>[6x]MPVERMRMRPWLEEQINSNTIPGLKWLNKEKKI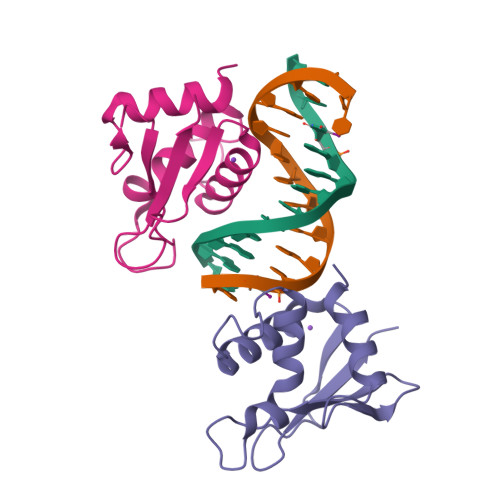FQIPWMHAARHGWDVEKDAPLFRNWAIHTGKHQPGIDKPDPKTWKANFRCAMNSLPDIEEVKDRSIKKGNNAFRVYRMLP>[24x]MRSATKLIKNVNINRCVQSNVVRSTSRLINNNSINTVRQFTSSSSSSFTSLFNNNNVNNTNIKYQRFYSSANDVVIKVPSMG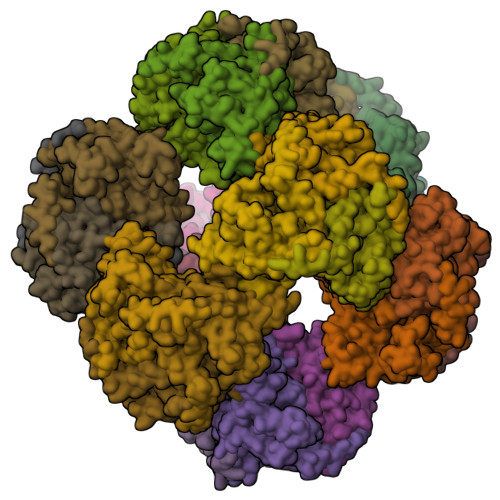DSISEGTIVAWTKNVGDSVRVDEVVCSIETDKVTIDINAPVSGTIVELFAKEGENVTVGNDLYKIAKGEVAAAPKVEAPKAAEAPKAAAPTPAPKAAETPKAAPAPKSEAPTPAPKSTTTTTSTGPSETRVKMTRIRQRTAQRLKDSQNTAAMLTTFNELDMSALMNMRKTYKDEFEKKHGVKFGFMSAFVKASTIALKEQPIVNASVEENDIVYHNNVNINVAVSAPRGLVVPVIRNCENLSFADIEKEIGRLSGLARNDALAIEDSIGGTFTISNGGVFGSMFGTPIINPPQSAILGMHAIKDRPYVVNGQVVVRPIMYLALTYDHRIIDGREAVTFLKKIKDVLENPERILLEL> GPKVPESGSMNLAAAERKKTGDLSVRSLHDIVKPEDFVLNSEHLTTVLVAVPKSLKSDFEKSYETLSKNVVPASASVIAEDAEYVLFNVHLFKKN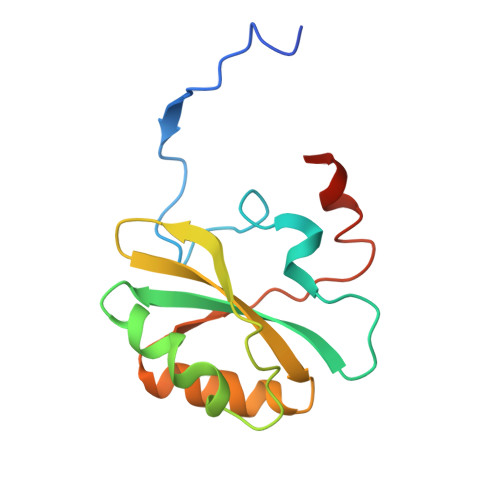VQEFTTAAREKKFIPREFNYSEELIDQLKKEHDSA Cytochrome P450 reductases (CPRs or CYPORs, EC 1.6.2.4) are diflavin oxidoreductases that supply electrons to type II cytochrome P450 monooxygenases (CYPs, EC 1.14.-.-). The structure is well conserved among the different kingdoms, possessing an N-terminal FMN-binding domain that is connected to a C-terminal FAD-binding domain via a linker region. The enzyme transfers electrons from NADPH in a typical order via flavin adenine dinucleotide (FAD) to flavin mononucleotide (FMN), which ultimately shuttles the electrons to the protein acceptors. Analysis of the CtCPR sequence revealed the presence of a single membrane-spanning region comprising the first 22 amino acids of the protein and in an attempt to produce more soluble CPR, a truncated, untagged version (Δ2–22) of the enzyme was expressed in E. coli.

The X-ray structures of CtCPR were solved with and without the cofactor, NADPH, at resolutions of 1.5 Å and 2.1 Å, respectively. Both structures were obtained in the closed conformation wherein the FMN-binding, flavodoxin-like domain interacts with the FAD and NADP- binding, ferredoxin-NADP+ reductase (FNR) like domain. In this conformation, the FMN and FAD moieties are in close proximity (~4.3 Å between the 7-methyl groups and ~3.6 Å between the 8-methyl groups), allowing direct electron transfer between the flavins. Even though only 22 residues were truncated at the N-terminus, density was only observed from residue 45, suggesting a relatively long flexible N-terminal region. Electron densities for both the FMN and FAD were well defined. The FMN-binding topology is conserved among the different CPRs, with the isoalloxazine ring hydrogen-bonded to backbone atoms in addition to some water-mediated hydrogen bonds. The FAD is bound in a fashion similar to that of yCPR where, in contrast to that observed for rCPR and hCPR, the adenosine moiety is buried, sandwiched between Pro364 and Val470, and hydrogen-bonded via N6A to the side chain oxygen of Asn406 and the main chain carbonyl oxygen of Phe405, in addition to various water-mediated contacts to other main chain atoms. Apart from the direct hydrogen bond formed with the side chain of Ser441, the isoalloxazine ring of FAD is mostly hydrogen-bonded to main-chain carbonyl and amine groups. The interface of the FMN and FAD-binding domains are stabilized with various salt-bridges and extensive hydrogen bonding networks, suggesting strong interactions between the domains. No differences were detected between the two structures, with the exception of the presence of the 3′-phosphate-adenosine-5′-diphosphate part of NADPH, which, in contrast to the FMN and FAD cofactors, is bound through mostly side chain interactions.

>MALDKLDLYVIITLVVAVAAYFAKNQFLDQPQDTGFLNTDSGSNSRDVLSTLKKNNKNTLLLFGSQTGTAEDYANKLSRELHSRFGLKTMVADFADYDWDNFGDITEDILVFFIVATYGEGEPTDNADEFHTWLTEEADTLSTLRYTVFGLGNSTYEFFNAIGRKFDRLLSEKGGDRFAEYAEGDDGTGTLDEDFMAWKDNVFDALKNDLNFEEKELKYEPNVKLTERDDLSAADSQVSLGEPNKKYINSEGIDLTKGPFDHTHPYLARITETRELFSSKERHCIHVEFDISESNLKYTTGDHLAIWPSNSDENIKQFAKCFGLEDKLDTVIELKALDSTYTIPFPTPITYGAVIRHHLEISGPVSRQFFLSIAGFAPDEETKKTFTRLGGDKQEFATKVTRRKFNIADALLYSSNNTPWSDVPFEFLIENIQHLTPRYYSISSSSLSEKQLINVTAVVEAEEEADGRPVTGVVTNLLKNIEIAQNKTGEKPLVHYDLSGPRGKFNKFKLPVHVRRSNFKLPKNSTTPVILIGPGTGVAPLRGFVRERVQQVKNGVNVGKTLLFYGCRNSNEDFLYKQEWAEYASVLGENFEMFNAFSRQDPSKKVYVQDKILENSQLVHELLTEGAIIYVCGDASRMARDVQTTISKIVAKSREISEDKAAELVKSWKVQNRYQEDVW[2x]>HMLGKIALEEAFALPRFEEKTRWWASLFSTDAETHVKEITDINKIRIEHADKHGVGYQILSYTAPGVQDIWDPVEAQALAVEINDYIAEQVRVNPDRFGAFATLSMHNPKEAADELRRCVEKYGFKGALVNDTQRAGPDGDDMIFYDNADWDIFWQTCTELDVPFYMHPRNPTGTIYEKLWADRKWLVGPPLSFAHGVSLHVLGMVTNGVFDRHPK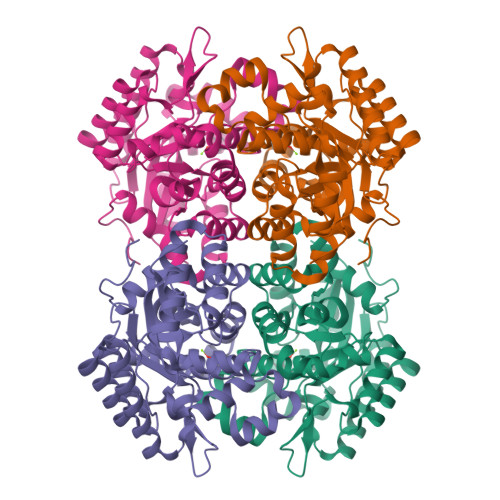LQIIMGHLGEHVPFDMWRINHWFEDRKKLLGLAETCKKTIRDYFAENIWITTSGHFSTTTLNFCMAEVGSDRILFSIDYPFETFSDACEWFDNAELNGTDRLKIGRENAKKLFKLDSYKDSSA[2x]>GPNPYERGPDPTEDSIEAIRGPFSVATERVSSFASGFGGGTIYYPRETDEGTFGAVAVAPGFTASQGSMSWYGERVASHGFIVFTIDTNTRLDAPGQRGRQLLAALDYLVERSDRKVRERLDPNRLAVMGHSMGGGGSLEATVMRPSLKASIPLTPWHLDKTWGQVQVPTFIIGAELDTIAPVSTHAKPFYESLPSSLPKAYMELCGATHFAPNIPNTTIAKYVISWLKRFVDEDTRYSQFLCPN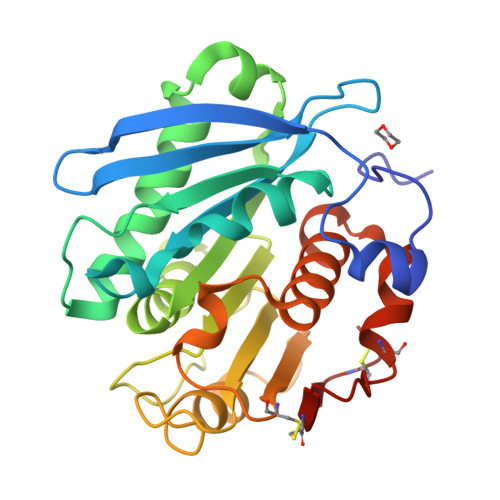PTDRAICEYRSTCPYKLN[2x]>[2x]PLHMSISNFQFPYTIEETAITETALWQCFDGTRKADSLPVTVFKAKRSPENESLILNAVHKSKILKIPGLCTVLETFDSDPQSTFI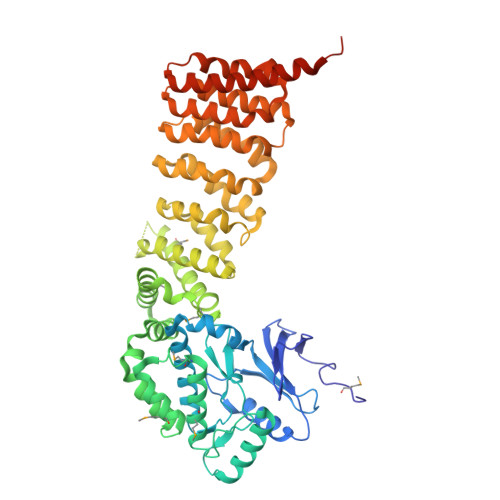VTERVVPFPWDNLGSLSQNKFGVELGISQLLATLGFLKNFVLGTLSKDSVFINIKGEWVLFGLELCSSKEGLSAFEFASRARSYYNIIGSQLPCEDPNTIDSMGLGLLIKSLMAPSCLPKDWIVNVNMISDGKITIENFRKRLENTETWRSNPLINFYQELRELHIKDPQGKLVVMSNLENLYLESREIFRNLTPGMIENFIIPELCEIIKLLMTQSISSAASPIGMNFNASHKLVPFLAIVLDLTSETNTFPVGFNDLITQSFKLPDRQVRFLLLIYLPKLIGPLSKSEISSRIYPHFIQGLTDSDATLRLQTLKTIPCIVSCLTERQLNNELLRFLAKTQVDSDVEIRTWTVIIISKISTILSTSVGNRSNILATAFTKSLKDPQVKPRLAALYGLEKSIELFDVNTIANKILTVIAPGLLDKSPIVRGRAKILFEEYLEKLEKEAQLIQTNDSTADSEDVKDIDFENYGCD> MKFYTISSKY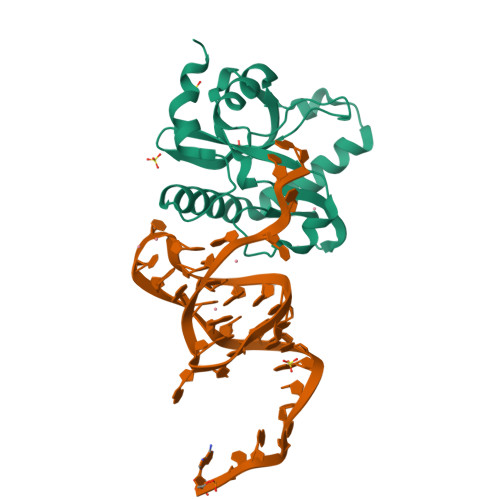IEYLKEFDDKVPNSEDPTYQNPKAFIGIVLEIQGHKYLAPLTSPKKWHNNVKESSLSCFKLHENGVPENQLGLINLKFMIPIIEAEVSLLDLGNMPNTPYKRMLYKQLQFIRANSDKIASKSDTLRNLVLQGKMQGTCNFSLLEEKYRDFGKEAEDTEEGE> MNITKPFPLPTGYFGIPLGLAALSLAWFHLENLFPAARMVSDVLGIVASAVWILFILMYAYKLRYYFEEVRAEYHSPVRFSFIALIPITTMLVGDILYRWNPLIAEVLIWIGTIGQLLFSTLRVSELWQGGVFEQKSTHPSFYLPAVAANFTSASSLALLGYHDLGYLFFGAGMIAWIIFEPVLLQHL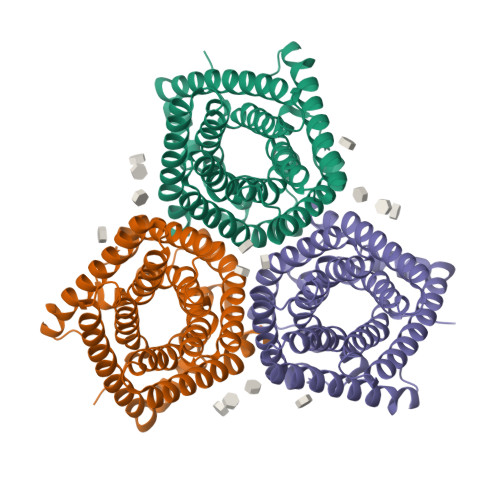RISSLEPQFRATMGIVLAPPFVCVSAYLSINHGEVDTLAKILWGYGFLQLFFLLRLFPWIVEKGLNIGLWAFSFPLASMANSATAFYHGNVLQGVSIFAFVFSNVMIGLLVLMTIYKLTKGQFFLK1-methylethyl 3-[(3,4-difluorophenyl)carbonyl]-1,1-dimethyl-1,2,3,6-tetrahydroazepino[4,5-b]indole-5-carboxylate 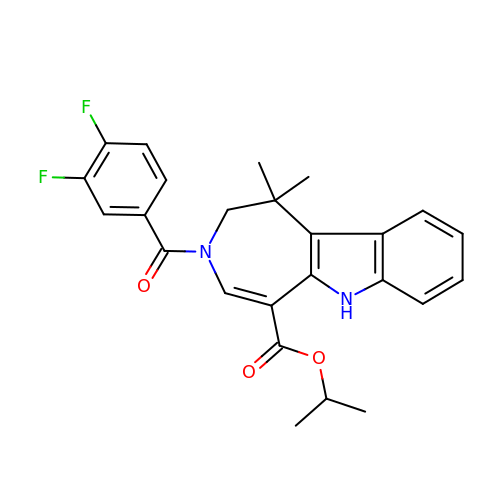| C25 H24 F2 N2 O3 | INASOKQDNHHMRE-UHFFFAOYSA-N> LTLGNTTSSVILTNYMDTQYYGEIGIGTPPQTFKVVFDTGSSNVWVPSSKCSRLYTACVYHKLFDASDSSSYKHNGTELTLRYSTGTVSGFLSQDIITVGGITVTQMFGEVTEMPALPFMLAEFDGVVGMGFIEQAIGRVTPIFDNIISQGVLKEDVFSFYYNRDSENSQSLGGQIVLGGSDPQHYEGNF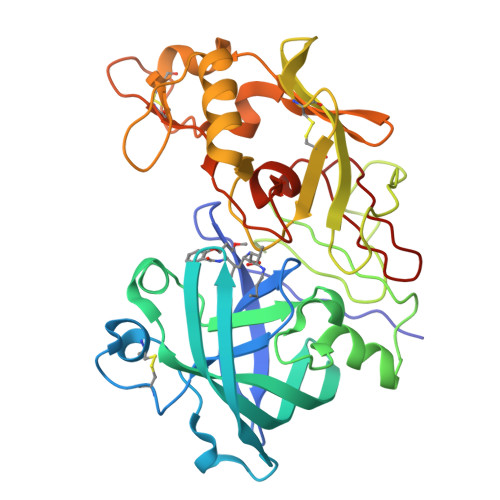HYINLIKTGVWQIQMKGVSVGSSTLLCEDGCLALVDTGASYISGSTSSIEKLMEALGAKKRLFDYVVKCNEGPTLPDISFHLGGKEYTLTSADYVFQESYSSKKLCTLAIHAMDIPPPTGPTWALGATFIRKFYTEFDRRNNRIGFALAR Polyketide synthase 13 (Pks13) of Mycobacterium tuberculosis, the bacterial organism causing tuberculosis, catalyses the last step of mycolic acid synthesis prior to export to and assembly in the cell wall. Pks13 is an iterative type I Pks composed of a sequence of catalytic and acyl carrier protein (ACP) domains separated by non-globular linker regions. Sandwiched between the functional ACPs are the central ketoacyl synthase (KS) and acyltransferase (AT) domains, which facilitate the condensation reaction, while the TE domain at the C-terminus loads the newly formed mycolate onto a trehalose. Due to its essentiality, Pks13 is a target for several novel anti-tubercular inhibitors, but its 3D structure and catalytic reaction mechanism remain to be fully elucidated.

Here, we report the molecular structure of the catalytic core domains of M. tuberculosis Pks13 (Mt-Pks13), determined by transmission cryo-electron microscopy (cryoEM) to a resolution of 3.4 Å. We observed a homodimeric assembly comprising the ketoacyl synthase (KS) domain at the centre, mediating dimerization, and the acyltransferase (AT) domains protruding in opposite directions from the central KS domain dimer. The structural model covers residues 106–550 and 596–1073 of the amino acid sequence of Mt-Pks13 for both monomers. The central KS domain dimer is resolved best, with local resolution down to 3.2 Å, while the distal ends of the AT domains show a spatial resolution of around 5 Å. Analysis of the KS dimer interface using PISA indicates a buried surface area of ~3500 Å2 per monomer. Reversible self-association aligns with a largely polar character of the dimer interface, which includes a small set of salt bridge interactions and about 35 H-bonds across the interface, contrasting with few hydrophobic interactions. Despite the disordered linker sequence between the KS and AT domains (residues 551–595), a stable relative orientation of the KS and AT domains is maintained through their extensive non-covalent contact interface (~2900 Å2 of solvent-accessible surface area buried). The cryoEM structure of Mt-Pks13 was obtained without substrates or inhibitors present in the protein solution. Our cryoEM map shows continuous backbone density for both subunits in the region N-terminal to residue Asp118, which clearly indicates an extended conformation of the ACP-KS linker sequence rather than a turn. As a result, the ACP of chain A likely associates with the KS domain of the opposite subunit (and vice versa).

>[2x]MADVAESQENAPAERAELTVPEMRQWLRNWVGKAVGKAPDSIDESVPMVELGLSSRDAVAMAADIEDLTGVTLSVAVAFAHPTIESLATRIIEGEPETDLAGDDAEDWSRTGPAERVDIAIVGLSTRFPGEMNTPEQTWQALLEGRDGITDLPDGRWSEFLEEPRLAARVAGARTRGGYLKDIKGFDSEFFAVAKTEADNIDPQQRMALELTWEALEHARIPASSLRGQAVGVYIGSSTNDYSFLAVSDPTVAHPYAITGTSSSIIANRVSYFYDFHGPSVTIDTACSSSLVAIHQGVQALRNGEADVVVAGGVNALITPMVTLGFDEIGAVLAPDGRIKSFSADADGYTRSEGGGMLVLKRVDDARRDGDAILAVIAGSAVNHDGRSNGLIAPNQDAQADVLRRAYKDAGIDPRTVDYIEAHGTGTILGDPIEAEALGRVVGRGRPADRPALLGAVKTNVGHLESAAGAASMAKVVLALQHDKLPPSINFAGPSPYIDFDAMRLKMITTPTDWPRYGGYALAGVSSFGFGGANAHVVVREVLPRDVVEKEPEPEPEPKAAAEPAEAPTLAGHALRFDEFGNIITDSAVAEEPEPELPGVTEEALRLKEAALEELAAQEVTAPLVPLAVSAFLTSRKKAAAAELADWMQSPEGQASSLESIGRSLSRRNHGRSRAVVLAHDHDEAIKGLRAVAAGKQAPNVFSVDGPVTTGPVWVLAGFGAQHRKMGKSLYLRNEVFAAWIEKVDALVQDELGYSVLELILDDAQDYGIETTQVTIFAIQIALGELLRHHGAKPAAVIGQSLGEAASAYFAGGLSLRDATRAICSRSHLMGEGEAMLFGEYIRLMALVEYSADEIREVFSDFPDLEVCVYAAPTQTVIGGPPEQVDAILARAEAEGKFARKFATKGASHTSQMDPLLGELTAELQGIKPTSPTCGIFSTVHEGRYIKPGGEPIHDVEYWKKGLRHSVYFTHGIRNAVDSGHTTFLELAPNPVALMQVALTTADAGLHDAQLIPTLARKQDEVSSMVSTMAQLYVYGHDLDIRTLFSRASGPQDYANIPPTRFKRKEHWLPAHFSGDGSTYMPGTHVALPDGRHVWEYAPRDGNVDLAALVRAAAAHVLPDAQLTAAEQRAVPGDGARLVTTMTRHPGGASVQVHARIDESFTLVYDALVSRAGSESVLPTAVGAATAIAVADGAPVAPETPAEDADAETLSDSLTTRYMPSGMTRWSPDSGETIAERLGLIVGSAMGYEPEDLPWEVPLIELGLDSLMAVRIKNRVEYDFDLPPIQLTAVRDANLYNVEKLIEYAVEHRDEVQQLHEHQKTQTAEEIARAQAELLHGKVGKTEPVDSEAGVALPSPQNGEQPNPTGPALNVDVPPRDAAERVTFATWAIVTGKSPGGIFNELPRLDDEAAAKIAQRLSERAEGPITAEDVLTSSNIEALADKVRTYLEAGQIDGFVRTLRARPEAGGKVPVFVFHPAGGSTVVYEPLLGRLPADTPMYGFERVEGSIEERAQQYVPKLIEMQGDGPYVLVGWSLGGVLAYACAIGLRRLGKDVRFVGLIDAVRAGEEIPQTKEEIRKRWDRYAAFAEKTFNVTIPAIPYEQLEELDDEGQVRFVLDAVSQSGVQIPAGIIEHQRTSYLDNRAIDTAQIQPYDGHVTLYMADRYHDDAIMFEPRYAVRQPDGGWGEYVSDLEVVPIGGEHIQAIDEPIIAKVGEHMSRALGQIEADRTSEVGKQ> MAQNLKDLAGRLPAGPRGMGTALKLLLGAGAVAYGVRESVFTVEGGHRAIFFNRIGGVQQDTILAEGLHFRIPWFQYPIIYDIRARPRKISSPTGSKDLQMVNISLRVLSRPNAQELPSMYQRLGLDYEERVLPSIVNEVLKSVVAKFNASQLITQRAQVSLLIRRELTERAKDFSLILDDVAITELSFSREYTAAVEAKQVAQQEAQRAQFLVEKAKQE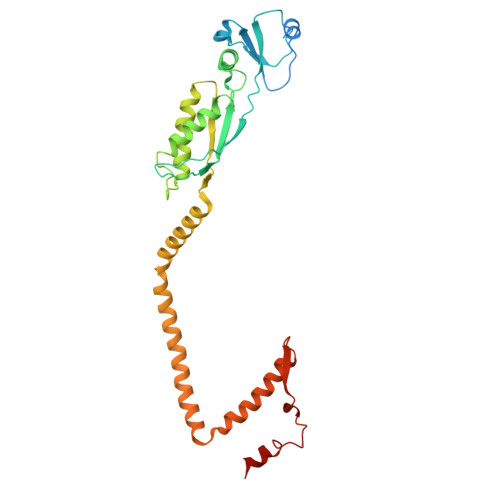QRQKIVQAEGEAEAAKMLGEALSKNPGYIKLRKIRAAQNISKTIATSQNRIYLTADNLVLNLQDESFTRGSDSLIKGKK> MVFSDQQLFEKVVEILKPFDLSVVDYEEICDRMGESMRLGLQKSTNEKSSIKMFPSYVTKTPNGTETGNFLALDLGGTNYRVLSVTLEGKGKSPRIQERTYCIPAEKMSGSGTELFKYIAETLADFLENNGMKDKKFDLGFTFSFPCVQKGLTHATLVRWTKGFSADGVEGHNVAELLQTELDKRELNVKCVAVVNDTVGTLASCALEDPKCAVGLIVGTGTNVAYIEDSSKVELMDGVKEPEVVINTEWGAFGEKGELDCWRTQFDKSMDIDSLHPGKQLYEKMVSGMYLGELVRHIIVYLVEQKILFRGDLPERLKVRNSLLTRYLTDVERDPAHLLYNTHYMLTDDLHVPVVEPIDNRIVRYACEMVVKRAAYLAGAGIACILRRINRSEVTVGVDGSLYKFHPKFCERMTDMVDKLKPKNTRFCL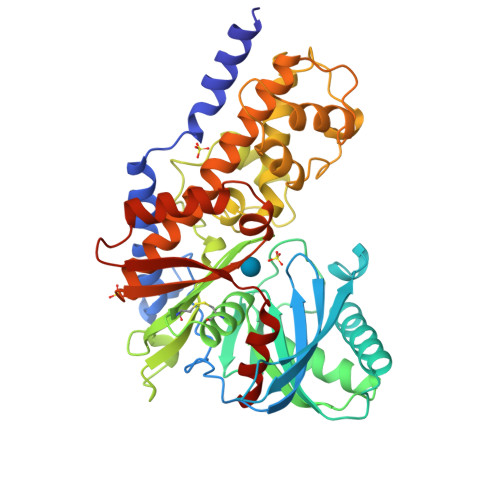RLSEDGSGKGAAAIAASCTRQN>GAMGSMWKRSEQMKIKSGKCNMAAAMETEQLGVEIFETADCEENIESQDRPKLEPFYVERYSWSQLKKLLADTRKYHGYMMAKAPHDFMFVKRNDPDGPHSDRIYYLAMSGENRENTLFYSEIPKTINRAAVLMLSWKPLLDLFQATLDYGMYSREEELLRERKRIGTVGIASYDYHQGSGTFLFQAGSGIYHVKDGGPQGFTQQPLRPNLVETSCPNIRMDPKLCPADPDWIAFIHSNDIWISNIVTREERRLTYVHNELANMEEDARSAGVATFVLQEEFDRYSGYWWCPKAETTPSGGKILRILYEENDESEVEIIHVTSPMLETRRADSFRYPKTGTANPKVTFKMSEIMIDAEGRIIDVIDKELIQPFEILFEGVEYIARAGWTPEGKYAWSILLDRSQTRLQIVLISPELFIPVEDDVMERQRLIESVPDSVTPLIIYEETTDIWINIHDIFHVFPQSHEEEIEFIFASECKTGFRHLYKITSILKESKYKRSSGGLPAPSDFKCPIKEEIAITSGEWEVLGRHGSNIQVDEVRRLVYFEGTKDSPLEHHLYVVSYVNPGEVTRLTDRGYSHSCCISQHCDFFISKYSNQKNPHCVSLYKLSSPEDDPTCKTKEFWATILDSAGPLPDYTPPEIFSFESTTGFTLYGMLYKPHDLQPGKKYPTVLFIYGGPQVQLVNNRFKGVKYFRLNTLASLGYVVVVIDNRGSCHRGLKFEGAFKYKMGQIEIDDQVEGLQYLASRYDFIDLDRVGIHGWSYGGYLSLMALMQRSDIFRVAIAGAPVTLWIFYDTGYTERYMGHPDQNEQGYYLGSVAMQAEKFPSEPNRLLLLHGFLDENVHFAHTSILLSFLVRAGKPYDLQIYPQERHSIRVPESGEHYELHLLHYLQENLGSRIAALKVI[3x]

Here we present the development and application of the Aerosol-Generator (AeGe), a new gentle soaking device that complements the humidity control and uses ultrasonic vibration to generate aerosols of ligands to soak reservoir-free protein crystals. The AeGe technique uses reservoir-free crystals under a temperature/humidity-controlled gas stream. In other words, ligands are directly soaked into protein crystals without being diluted in the crystallization drop. Two protein model systems confirm the advantages of using the AeGe method in challenging complex formation scenarios.

We tested the AeGe on dipeptidyl peptidase (DPP8) crystals using two ligands which evaded complex formation by regular soaking methods. Both 1G244 and the E67-interacting loop (EIL) peptide (SLRFLFEGQRIADNH) are inhibitors of DPP8 and DPP9. 1G244 is a model for a water-insoluble mol­ecule and the EIL peptide is a model for a low-affinity binder: neither forms complexes with DPP8 using classical soaking. Regardless of the low nM binding affinity of 1G244 for DPP8/9, the low solubility of the compound in aqueous solution might explain the lack of complex formation with DPP8. A pre-filled capillary with 10 mM 1G244 in 100% DMSO was positioned near the active surface of the AeGe. As the humidity decreased, both ligand and DMSO were concentrated in the crystal. The crystallographic structure of the AeGe-soaked DPP8–1G244 crystals was determined at 3.2 Å. We identified positive electron density in the active site corresponding to 1G244 [Fig. 7(a)]. The 1G244 molecule is fully visible. Importantly, the atoms of the fluoro­benzhydryl substituent occupy S2, but also overlap with S1′ and S2′.>MAHHHHHHMSRSETLFNNAQKHIPGGVNSPVRAFKSVGGTPLFFKHAEGAYVLDEDDKRYVDYVGSWGPMILGHSHPDVLDAVRRQLDHGLSYGAPTALEVEMADLVCSMVPSMEMVRMVSSGTEATMSAIRLARGYTGRDSIIKFEGCYHGHSDSLLVKAGSGALTFGVPNSPGVPAAFAKHTLTLPFNDIEAVRKTLGEVGKEVACIIVEPVAGNMNCVPPAPGFLEGLREACDEHGVVLIFDEVMTGFRVALGGAQAYYGVTPDLSTFGKIIGGGMPVGAFGGKREIMQQISPLGPVYQAGTLSGNPLAMAAGLTTLRLISRPGFHDELTAYTTRMLDGLQQRADAAGIPFVTTQAGGMFGLYFSGADAIVT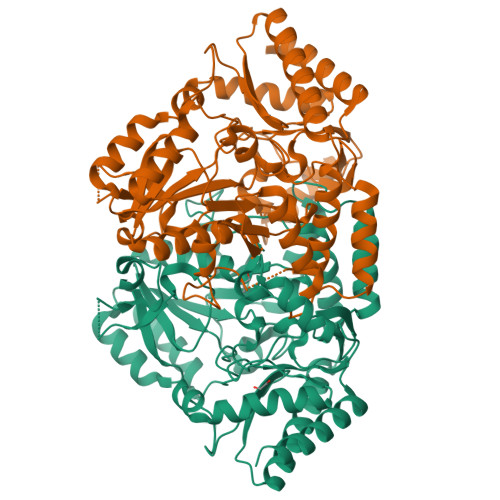FEDVMASDVERFKRFFHLMLDGGVYLAPSAFEAGFTSIAHGDKELEITLNAAEKAFAALK[6x]>[4x]SELWYTEKQTKNFGITMKVNKTLHTEQTEFQHLEMVETEEFGNMLFLDGMVMTSEKDE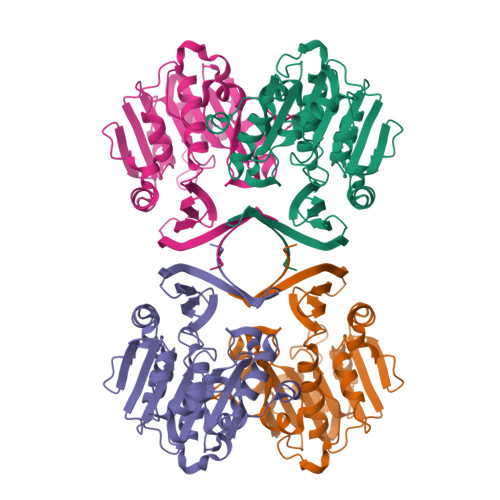FVYHEMVAHVPLFTHPNPEHVLVVGGGDGGVIREILKHPSVKKATLVDIDGKVIEYSKKFLPSIAGKLDDPRVDVQVDDGFMHIAKSENQYDVIMVDSTEPVGPAVNLFTKGFYAGIAKALKEDGIFVAQTDNPWFTPELITNVQRDVKEIFPITKLYTANIPTYPSGLWTFTIGSKKYDPLAVEDSRFFDIETKYYTKDIHKAAFVLPKFVSDLIK> PETTVLS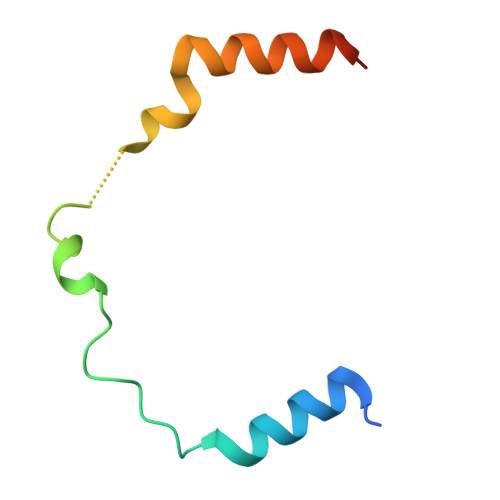GRDRLKRHREEVAGKVPIPDSWGKEGLLMGWMDFSTFDAAFTSSQIVSARAALMADSGHHHHHH> KLAFPRELRLLTPSQFTFVFQQPQRAGTPQITILGRLNSLGHPRIGLTVAKKNVRRAHERNRIKRLTRESFRLRQHELPAMDFVVVAKKGVADLDNRALSEALEKLWRRHCR

Ribonuclease P (RNase P) is an endonuclease whose primary role is to remove diverse 5′ leader sequences from precursor tRNAs (ptRNAs). Bacterial RNase P consists of a ~400 nucleotide P RNA and a single protein (rnpA, ~120 amino acids). RNase P recognizes the shape of the stacked acceptor and T-stems which span the two domains that together form a molecular ruler. In bacterial RNase P the 3′ RCCA of ptRNA pairs with a loop or internal bulge in the C-domain (L15), while a conserved adenosine in the catalytic core contacts an optimal U(−1) flanking the cleavage site 5′ to N(1).

To better understand how unwinding occurs and delineate the structural basis for such plasticity, we used cryo-electron microscopy (cryoEM) single particle analysis (SPA) to determine the structures of holoenzyme and ES* complexes formed with ptRNA_GG and ptRNA_AU. The ptRNA_AU substrate has the optimal consensus leader while ptRNA_GG contains the slowest dinucleotide sequence at N(−1)N(−2). Only a small percentage of ptRNA_AU dissociates during the entire time course. In both ptRNA_AU and ptRNA_GG bound complexes, the 5′ leader is positioned with the correct phosphodiester bond placed in the active site, while the 3′ RCCA is trapped in the L15 internal bulge loop of RNase P. When a smaller nucleobase occupies the N(−1) position of the leader sequence, as in the case of the ptRNA_AU-bound substrate, it forms a parallel stacking interaction with G1-C73 base pair of ptRNA and A248 of RNase P. The N(−2) position of the ptRNA leader stacks with A333 of RNase P in both the ptRNA_AU and ptRNA_GG complexes. At the U(−5), only map features for the phosphodiester backbone are observed in both AU_ES* and GG_ES* cryoEM maps. We observed a similar inner-sphere ion coordination of an MA ion at the G1 phosphate group in both ES* complexes. Notably, the distribution of the three classes identifies a significantly larger proportion of ptRNA-bound RNase P for the ptRNA_AU (~80% ES* complex) over ptRNA_GG (~46% ES* complex) dataset.>GAMEEETFYSVRMRASMNGSHEDGGKHISGGERLIPFHEMKHTVNALLEKGLSHSRGKPDFMQIQFEEVHESIKTIQPLPVHTNEVSCPE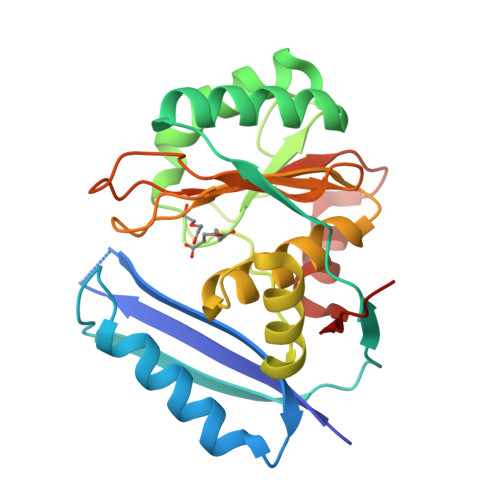EGQKLARLLLEKEGVSRDVIEKAYEQIPEWSDVRGAVLFDIHTGKRMDQTKEKGVRVSRMDWPDANFEKWALHSHVPAHSRIKEALALASKVSRHPAVVAELCWSDDPDYITGYVAGKKMGYQRITAMKEYGTEEGCRVFFIDGSNDVNTYIHDLEKQPILIEWEEDHDS[2x]> TLTEDLDAPQDTGNIENGAADNSPQPRTTFDYTGNPLPPDTKLENFFSFYRLLPMGGSGAPSLSFPADEGTIIPLNPINWLKGADVSGIAAMLSCFTYIAADLRITLRFSNPNDNPATMLVAFAPPGATIPLKPTRQMLSNFYMAEVPVSAATSTMVSFSIPYTSPLSAIPTSYFGWEDWSGTNFGQLSSGSWGNLMLIPSLSVDSAIPFDFQLSCWVAFGNFKAWVPRPPPPLPPLPTPAANAERTVAVIKQ;> GNSVTNIYGNGNNVTTDVGANGWAPTVSTGLGDGPVSASADSLPGRSGGASSEKTHTVSGS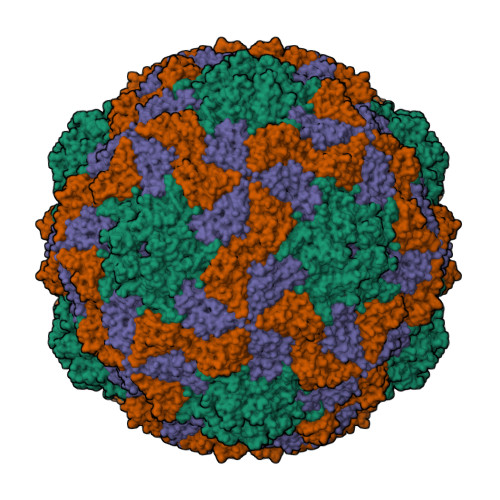SNKVGSRFSKWWEPAAARASESATDSAIEGIDAAGKAASKAITRKLDRPAAPSSTANPQPSLIALNPSATQSGNASILTGSTAPSLLAYPTATPVPLPNPDEPSQPGPSGDRTWLLDTVTWSQEFTRGWNIAGSNGMQWTGLESLIFPVSTDTNWTSTSSPTAYPLPFSFVRAYPDSSWAAMYNTHSMWNCGWRVQVTVNGSQFHAGALILYMVPEATTHAIQTARDNAGFVFPYVILNLYESNTATIEVPYISPTPNTSSGLHAPWTFYLQVLSPLNPPPSLPTSLSCSIYVTPVDSSFHGLRYLAPQ;> HWKTRAVPGAGTFGSAVAGQELPLCGVRAYYPPNAYIPAQVRDWLEFAHRPGLMATVPWTMADEPAERLGIFPVSPSAIAGTGAPISYVISLFSQWRGELAAHLLFTGSAQHYGRLVVCYTPAAPQPPSTMQEAMRGTYTVWDVNAASTLEFTIPFISNSYWKTVDVNNPDALLSTTGYVSIWVQNPLVGPHTAPASALVQAFISAGESFNVRLMQNPALTSQ> APGDPRENSNNHYDKILAHSRIRGRDQGPNVCALQQILGTKKKYFSTCKNWYKKSICGQKTTVLYECCPGYMRMEGMKGCPAVLPIDHVYGTLGIVGATTTQRYSDASKLREEIEGKGSFTYFAPSNEAWDNLDSDIRRGLESNVNVELLNALHSHMINKRMLTKDLKNGMIIPSMYNNLGLFINHYPNGVVTVNCARIIHGNQIATNGVVHVIDRVLTQIGTS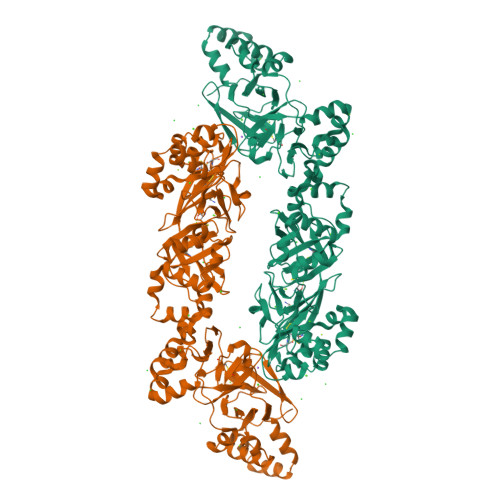IQDFIEAEDDLSSFRAAAITSDILEALGRDGHFTLFAPTNEAFEKLPRGVLERIMGDKVASEALMKYHILNTLQCSESIMGGAVFETLEGNTIEIGCDGDSITVNGIKMVNKKDIVTNNGVIHLIDQVLIPDSAKQVIELAGKQQTTFTDLVAQLGLASALRPDGEYTLLAPVNNAFSDDTLSMDQRLLKLILQNHILKVKVGLNELYNGQILETIGGKQLRVFVYRTAVCIENSCMEKGSKQGRNGAIHIFREIIKPAEKSLHEKLKQDKRFSTFLSLLEAADLKELLTQPGDWTLFVPTNDAFKGMTSEEKEILIRDKNALQNIILYHLTPGVFIGKGFEPGVTNILKTTQGSKIFLKEVNDTLLVNELKSKESDIMTTNGVIHVVDKLLYPAAAHHHHHHH> MKQKVVSIGDINVANDLPFVLFGGMNVLESRDLAMRICEHYVTVTQKLGIPYVFKASFDKANRSSIHSYRGPGLEEGMKIFQELKQTFGVKIITDVHEPSQAQPVADVVDVIQLPAFLARQTDLVEAMAKTGAVINVKKPQFVSPGQMGNIVDKFKEGGNEKVILCDRGANFGYDNLVVDMLGFSIMKKVSGNSPVIFDVTHALQCRDPFVAASGG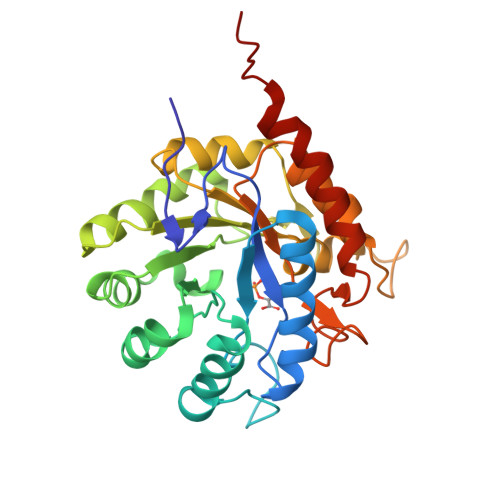RRAQVAELARAGMAVGLAGLFIEAHPDPEHAKCDGPSALPLAKLEPFLKQMKAIDDLVKGFEELDTSK>[2x]GPMGTDWPVYHRIDGPIVMIGFGSIGRGTLPLIERHFAFDRSKLVVIDPSDEARKLAEARGVRFIQQAVTRDNYRELLVPLLTAGPGQGFCVNLSVDTSSLDIMELARENGALYIDTVVEPWLGFYFDPDLKPEARSNYALRETVLAARRNKPGGTTAVSCCGANPGMVSWFVKQALVNLAADLGVTGEEPTTREEWARLAMDLGVKGIHIAARDTQRASFPKPFDVFVNTWSVEGFVSEGLQPAELGWGTFERWMPDNARGHDSGCGAGIYLLQPGANTRVRSWTPTAMAQYGFLVTHNESISIADFLTVRDAAGQAVYRPTCHYAYHPCNDAVLSLHEMFGSGKRQSDWRILDETEIVDGIDELGVLLYGHGKNAYWYGSQLSIEETRRIAPDQNATGLQVSSAVLAGMVWALENPNAGIVEADDLDFRRCLEVQTPYLGPVVGVYTDWTPLAGRPGLFPEDIDTSDPWQFRNVLVRD

Bacterial HSS is mostly found in α-proteobacteria and in some β- and γ-proteobacteria, including pathogenic strains such as Legionella pneumophila, Brucella spp. and various P. aeruginosa strains, including PA7 and PA14. It catalyzes the conversion of two molecules of putrescine (PUT; 1,4-diaminobutane) into one molecule of sym-homospermidine [HSP; bis(4-aminobutyl)amine] as the main reaction along with several side reactions (Ober et al., 1996; Böttcher et al., 1994). Bacterial HSS is NAD+-dependent, active at neutral to basic pH with an optimum at pH ∼8.8, and shows increased activity in the presence of 50 mM potassium ion. BvHSS forms a dimer, with each subunit containing a boot-shaped substrate-binding pocket between an NAD(P)-binding Rossmann-like domain and an HSS-like domain. The cofactor NAD+ is bound as a prosthetic group in the binding pocket with its nicotinamide ring being part of the active site.

Krossa and coworkers identified three binding sites for the amino groups of reaction components within the substrate-binding pocket. Assuming the amino groups of the reaction components to be protonated at neutral to slightly basic pH, the ‘innermost’ N atoms of PUT (N1) and of HSP (N01) mainly bind via a salt bridge to Glu210 and, in addition, via a hydrogen bond to Asn162 at the ‘inner amino site’. Following a similar approach to probe the role of BvHSS residue Glu210, the E210A, E210Q and E210K variants were examined and were found to be inactive. Superimposition of the variant structures onto the wild-type structure revealed nearly identical locations of all residues in the binding pocket, including the wild-type and variant residues Glu210 and Gln210. These findings convincingly demonstrate the indispensable need for a negative charge at position 210 to stabilize the positively charged amino groups of the reaction component at the ‘inner amino site’.> ATITQDTPINQIFTDTALAEKMKTVLGKTNVTDTVSQTDLDQVTTLQADRLGIKSIDGVEYLNNLTQINFSNNQLTDITPLKNLTKLVDILMNNNQIADITPLANLTNLTGLTLFNNQITDIDPLKNLTNLNRLELSSNTISDISALSGLTSLQQLNFSSNQVTDLKPLANLTTLERLDISSNKVSDISVLAKLTNLESLIATNNQISDITPLGILTNLDELSLNGNQLKDIGTLASLTNLTDLDLANNQISNLAPLSGLTKLTELKLGANQISNISPLAGLTALTNLELNENQLEDISPISNLKNLTYLTLYFNNISDISPVSSLTKLQRLFFYNNKVSDVSSLANLTNINWLSAGHNQISDLTPLANLTRITQLGLNDQAWTNAPVNYKANVSIPNTVKNVTGALIAPATISDGGSYTEPDITWNLPSYTNEVSYTFSQPVTIGKGTTTFSGTVTQPLKA;> GPLGSWVIPPISCPENEKGPFPKNLVQIKSNKDKEGKVFYSITGQGADTPPVGVFIIERETGWLKVTEPLDRERIATYTLFSHA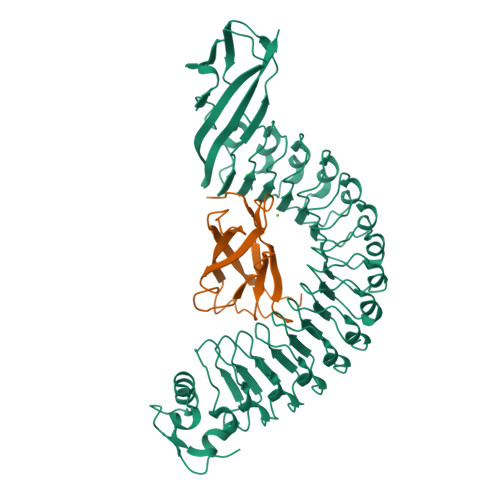VSSNGNAVEDPMEILITVTDQNDN> MSGLPLISRRRLLTAMALSPLLWQMNTAHAAAIDPNRIVALEWLPVELLLALGIVPYGVADTINYRLWVSEPPLPDSVIDVGLRTEPNLELLTTMRPSFMVWSAGYGPSPEMLA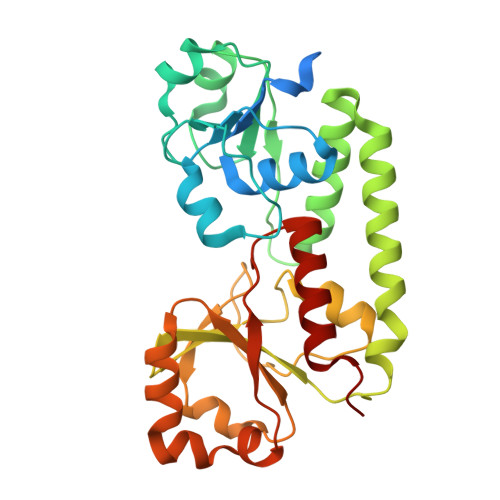RIAPGRGFNFSDGKQPLAMARKSLTEMADLLNLQSAAETHLAQYEDFIRSMKPRFVKRGARPLLLTTLIDPRHMLVFGPNSLFQEILDEYGIPNAWQGETNFWGSTAVSIDRLAAYKDVDVLCFDHDNSKDMDALMATPLWQAMPFVRAGRFQRVPAVWFYGATLSAMHFVRVLDNAIGGKA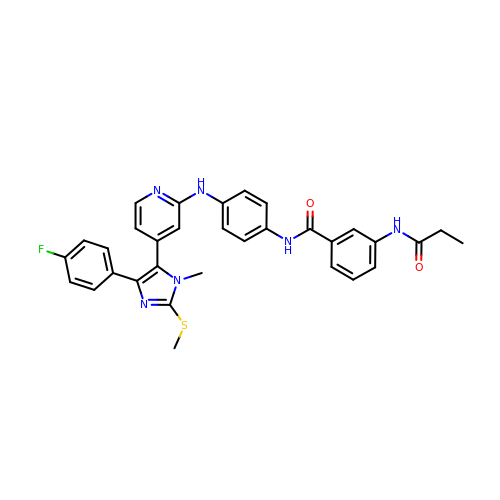N-[4-[[4-[5-(4-fluorophenyl)-3-methyl-2-methylsulfanyl-imidazol-4-yl]pyridin-2-yl]amino]phenyl]-3-(propanoylamino)benzamide | C32 H29 F N6 O2 S | UKLFJWKRYNOIGW-UHFFFAOYSA-N> PRSLQNRNTKNLSLDIAALH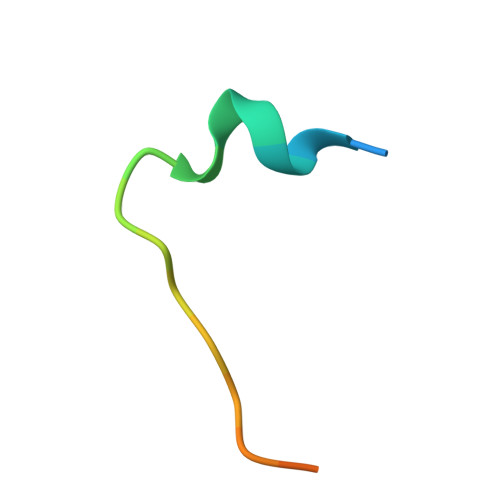P PHOSPHOMETHYLPHOSPHONIC ACID GUANYLATE ESTER | C11 H18 N5 O13 P3 | 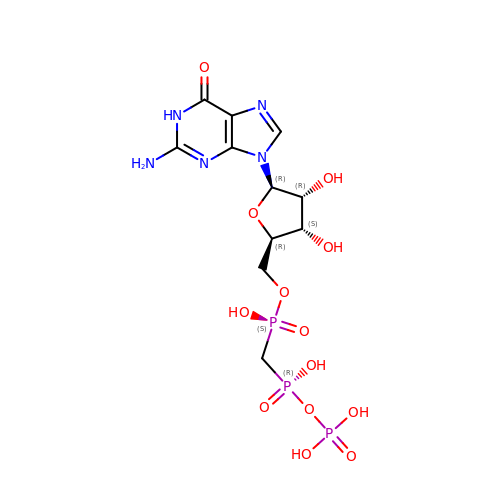GXTIEXDFEKYVGY-KQYNXXCUSA-N> GSSGSSGCVNQVLTAKEIKRQEAIFELSQGEEDLIEDLKLAKKAYHDPMLKLSIMTEQELNQIFGTLDSLIPLHEELLSQLRDVRKP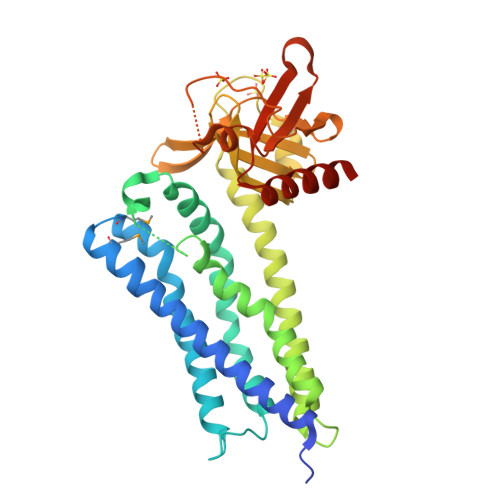DGSTEHVGPILVGWLPCLSSYDSYCSNQVAAKALLDHKKQDHRVQDFLQRCLESPFSRKLDLWNFLDIPRSRLVKYPLLLREILRHTPNDNPDQQHLEEAINIIQGIVAEINTKTGESECRYYKERLLYLEEGQKDSLIDSSRVLCCHGELKNNRGVKLHVFLFQEVLVITRAVTHNEQLCYQLYRQPIPVKDLTLEDLQDGEVRLGGSLRGAFSNNERVKNFFRVSFKNGSQSQTHSLQANDTFNKQQWLNCIRQAKESGPSSG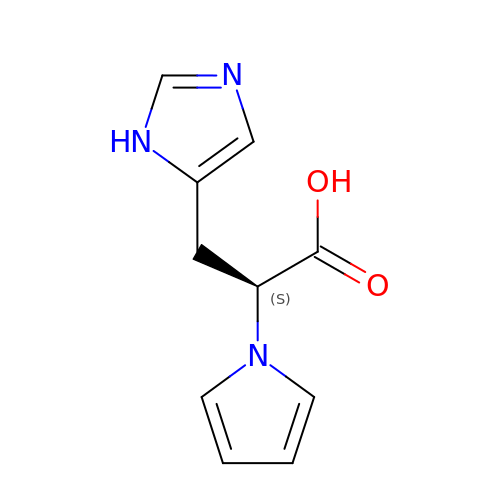(2S)-3-(1H-imidazol-5-yl)-2-(1H-pyrrol-1-yl)propanoic acid | C10 H11 N3 O2 | XTGWWGRMXKSWQM-VIFPVBQESA-N>MPCPKEDTPNSVWEPAKAKYVFRDVVQITCLDGFEVVEGRVGATSFYSTCQSNGKWSNSKLKCQPVDCGIPESIENGKVEDPESTLFGSVIRYTCEEPYYYMENGGGGEYHCAGNGSWVNEVLGPELPKCVPVCGVPREPFEEKARAIGGSDADIKNFPWQVFFDNPWAGGALINEYWVLTAAHVVEGNREPTMYVGSTSVQTSRLAKSKMLTPEHVFIHPGWKLLEVPEGRTNFDNDIALVRLKDPVKMGPTVSPICLPGTSSDYNLMDGDLGLISGWGRTEKRDRAVRLKAARLPVAPLRKCKEVKVEKPTADAEAYVFTPNMICAGGEKGMDSCKGDSGGAFAVQDPN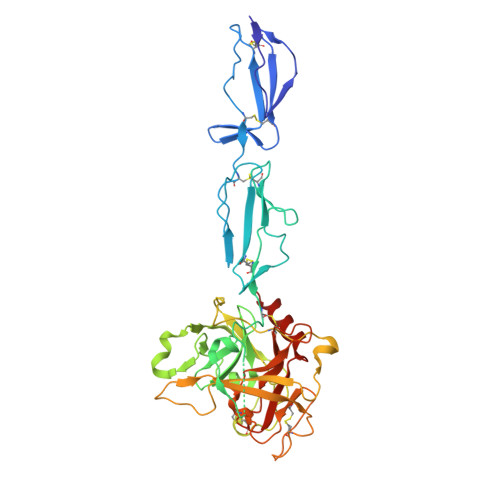DKTKFYAAGLVSWGPQCGTYGLYTRVKNYVDWIMKTMQENSTPRED[2x]>MTELSPTALDPTELRSSLDKPFGTNRVIADDAMMADSITPAQYRYHHGSRVRPVNWNNIVDDKDLDVWNRLIANFWLPEKVPLSNDIPSWRSLTDLERKTTTRVFTGLTLLDTSQATIGELCQIEHARTEHEQAIYTNIAFMQSIHARSYSSIFSTLCSSEEIDEAYRWAVGNDVLQQRVTTVLCEYESEDPLKRKIAATMLSSLLLYAGFYLPLYFASRGKMMNTADMIRLILRDKAIHGYYSGYKFQRGLELRSENDKKNLEKFTMNLLDTLYDLEVEYSGQIYEGFDFHDDVFDFVRYNANKALMNLGYPAKYSEEETHVSPEILAALSPAADENHDFFSGSGSSYIMGKSVETDDDDWDF[4x]

Class I ribonucleotide reductases (RNRs) convert ribonucleotides into deoxyribonucleotides under oxic conditions. The R2 subunit provides a radical required for catalysis conducted by the R1 subunit. The discovery of a metal-free R2 defined the new RNR subclass Ie. In R2e, three of the otherwise strictly conserved metal-binding glutamates in the active site are substituted.

We first crystallized R2 expressed alone and solved the structure of unmodified BvR2eQSK (BvR2QSK-tyr) at 1.8 Å resolution in space group P3121 with four monomers in the asymmetric unit forming two homodimers that correspond to the physiological active form of other R2 subunits. Of the 364 amino acids, residues 6 to 333 could be modelled in the electron density. The N-terminus is extended and contacts the second monomer of the dimer, creating a large interaction surface of about 4300 Å2 and forming 6 salt bridges between the monomers. The typical interaction surface for published structures of R2 is between 1000 and 2500 Å2; the area for BvR2QSK is therefore much larger. The active site residues are well-defined. There are no metal ions observed in the active site. Residues Y150, H146, H240 and D112 are in the same position as in other R2bs. The remaining glutamates that usually bind metals in the site are as expected from the sequence substituted to Q143, S203 and K237. The position of Mn1 is occupied by the ε-ammonium group of K237 and in the position of Mn2 a well-defined water is bound. The DOPA containing R2eQSK can support ribonucleotide reduction in vitro while the unmodified protein cannot.>ILGGREAEAHARPYMASVQLNGAHLCGGVLVAEQWVLSAAHCLEDAADGKVQVLLGAHSLSQPEPSKRLYDVLRAVPHPDSQPDTIDHDLLLLQLSEKATLGPAVRPLPWQRVDRDVAPGTLCDVAGWGIVNHAGRRPDSLQHVLLPVLDRA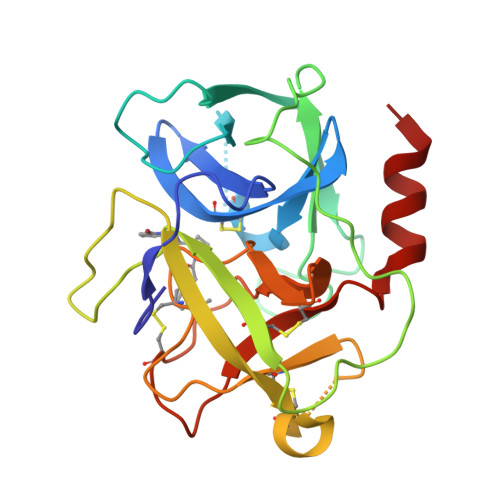TCNRRTHHDGAITERLMCAESNRRDSCKGDSGGPLVCGGVLEGVVTSGSRVCGNRKKPGIYTRVASYAAWIDSVLASA[4x]>[7x]ADSDINIKTGTTDIGSNTTVKTGDLVTYDKENGMHKKVFYSFIDDKNHNKKLLVIRTKGTIAGQYRVYSEEGANKSGLAWPSAFKVQLQLPDNEVAQISDYYPRNSIDTKEYFSTLTYGFNGNVTGDDTGKIGGLIGANVSIGHTLKYVQP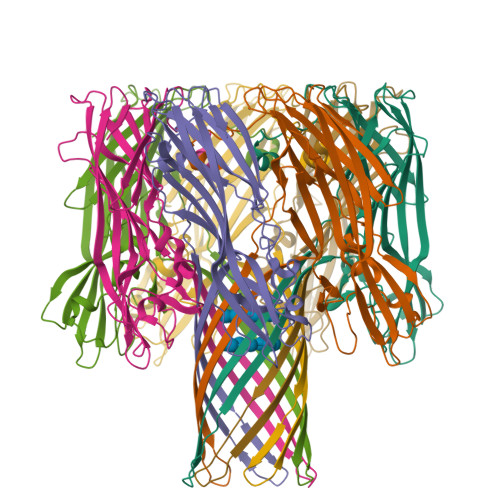DFKTILESPTDKKVGWKVIFNNMVNQNWGPYDRDSWNPVYGNQLFMKTRNGSMKAADNFLDPNKASSLLSSGFSPDFATVITMDRKASKQQTNIDVIYERVRDDYQLHWTSTNWKGTNTKDKWTDRSSERYKIDWEKEEMTN>THLRPYETLGAHADTMDGVTGTRFSVWAPNARRVSVVGQFNYWDGRRHPMRLRKESGIWELFIPGAHNGQLYKYEMIDANGNLRLKSDPYAFEAQMRPETASLICGLPEKVVQTEERKKANQFDAPISIYEVHLGSWRRHTDNNFWLSYRELADQLVPYAKWMGFTHLELLPINEHPFDGSWGYQPTGLYAPTRRFGTRDDFRYFIDAAHAAGLNVILDWVPGHFPTDDFALAEFDGTNLYEHSDPREGYHQDWNTLIYNYGRREVSNFLVGNALYWIERFGIDALRVDAVASMIYRDYSRKEGEWIPNEFGGRENLEAIEFLRNTNRILGEQVSGAVTMAEESTDFPGVSRPQDMGGLGFWYKWNLGWMHDTLDYMKLDPVYRQYHHDKLTFGILYNYTENFVLPLSHDEVVHGKKSILDRMPGDAWQKFANLRAYYGWMWAFPGKKLLFMGNEFAQGREWNHDASLDWHLLEGGDNWHHGVQRLVRDLNLTYRHHKAMHELDFDPYGFEWLVVDDKERSVLIFVRRDKEGNEIIVASNFTPVPRHDYRFGINQPGKWREILNTDSMHYHGSNAGNGGTVHSDEIASHG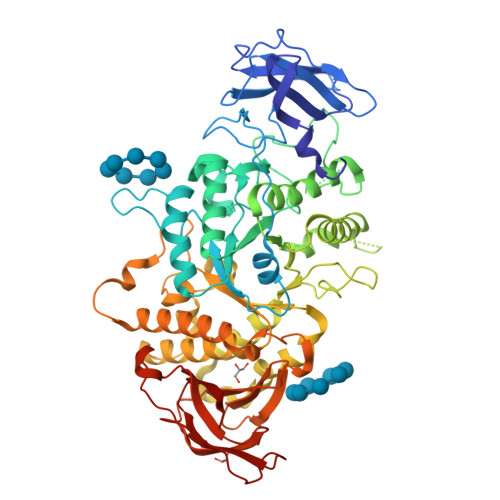RQHSLSLTLPPLATIWLVREAE[4x]> DEKYVNSIWDLLKNAIQEIQRKNNSGLSFEELYRNAYTMVLHKHGEKLYTGLREVVTEHLINKVREDVLNSLNNNFLQTLNQAWNDHQTAMVMIRDILMYMDRVYVQQNNVENVYNLGLIIFRDQVVRYGCIRDHLRQTLLDMIARERKGEVVDRGAIRNACQ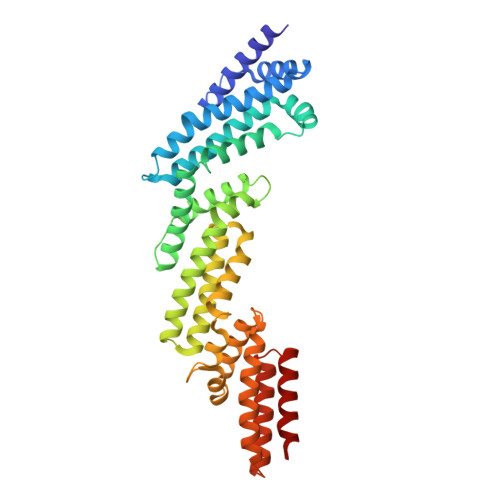MLMILGLEGRSVYEEDFEAPFLEMSAEFFQMESQKFLAENSASVYIKKVEARINEEIERVMHCLDKSTEEPIVKVVERELISKHMKTIVEMENSGLVHMLKNGKTEDLGCMYKLFSRVPNGLKTMCECMSSYLREQGKALVSEEGEGKNPVDYRQGLDDLKSRFDRFLLESFNNDRLFKQTIAGDFEYFLNLN>[2x]MGYLNNVTGYREDLLANRAIVKHGNFALLTPDGLVKNIIPGFENCDATILSTPKLGASFVDYLVTLHQNGGNQQGFGGEGIETFLYVISGNITAKAEGKTFALSEGGYLYCP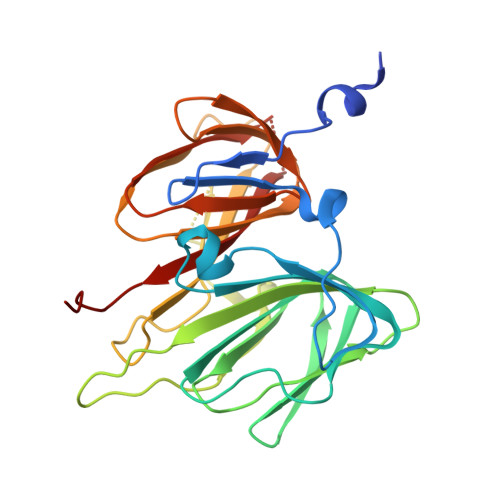PGSLMTFVNAQAEDSQIFLYKRRYVPVEGYAPWLVSGNASELERIHYEGMDDVILLDFLPKELGFDMNMHILSFAPGASHGYIETHVQEHGAYILSGQGVYNLDNNWIPVKKGDYIFMGAYSLQAGYGVGRGEAFSYIYSKDCNRDVEI2-(3-chloro-2-methylanilino)pyridine-3-carboxylic acid | C13 H11 Cl N2 O2 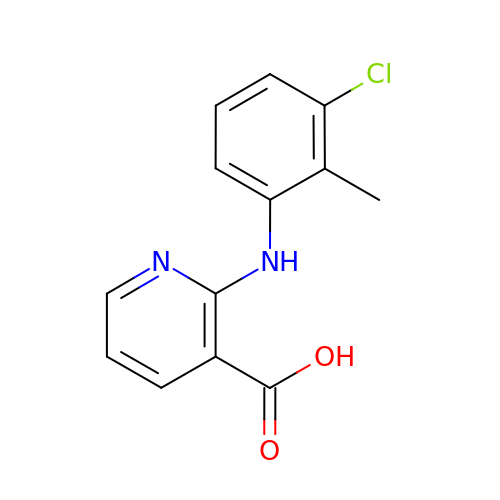| CLOMYZFHNHFSIQ-UHFFFAOYSA-N We now report characterization of CRT0063465, a novel pyrazolopyrimidine compound that emerged from cell-based screens of telomere signaling. CRT0063465 targets the nucleotide binding site of glycolytic enzyme phosphoglycerate kinase 1 (PGK1). We show here that DJ1 and PGK1 form a previously unknown complex in cells. We show that both proteins bind TRF2 and telomeric DNA.

To investigate binding modes of the unlabeled parent compound CRT0063465 to these proteins, X-ray crystallography was performed. A PGK1- CRT0063465 co-structure was obtained at 1.9 Å resolution. Binding is perpendicular to the nucleotide binding site. The compound bromo-phenyl moiety occupies the same position as the nucleotide adensosine ring. The aryl ring is co-planar with the pyrrolopyrimidine scaffold and the para-substituted bromine engages a deep hydrophobic pocket. The carboxylate moiety on the distal end of the pryrazolopyrimidine scaffold is solvent-exposed and does not interact via any polar or hydrogen bonding interactions with PGK1. CRT0063465 makes no hydrogen-bonding hinge region interactions. This mode would be unusual for an ATP-competitive kinase inhibitor, which normally bind mainly through this mechanism. CRT0063465-bound PGK1 domains are locked in the “open” conformation, each interacting in a clamp-like fashion with a single DJ1 monomer on opposite sides of the complex, giving 2:2:2 CRT0063465:DJ1:PGK1 stoichiometry.

> GSHMSLSNKLTLDKLDVKGKRVVMRVDFNVPMKNNQITNNQRIKAAVPSIKFCLDNGAKSVVLMSHLGRPDGVPMPDKYSLEPVAVELKSLLGKDVLFLKDCVGPEVEKACANPAAGSVILLENLRFHVEEEGKGKDASGNKVKAEPAKIEAFRASLSKLGDVYVNDAFGTAHRAHSSMVGVNLPQKAGGFLMKKELNYFAKALESPERPFLAILGGAKVADKIQLINNMLDKVNEMIIGGGMAFTFLKVLNNMEIGTSLFDEEGAKIVKDLMSKAEKNGVKITLPVDFVTADKFDENAKTGQATVASGIPAGWMGLDCGPESSKKYAEAVTRAKQIVWNGPVGVFEWEAFARGTKALMDEVVKATSRGCITIIGGGDTATCCAKWNTEDKVSHVSTGGGASLELLEGKVLPGVDALSNI> ACDVSIEGNDSMQFNTKSIVVDKTCKEFTINLKHTGKLPKAAMGHNVVVSKKSDESAVATDGMKAGLNNDYVKAGDERVIAHTSVIGGGETDSVTFDVSKLKEGEDYAFFCS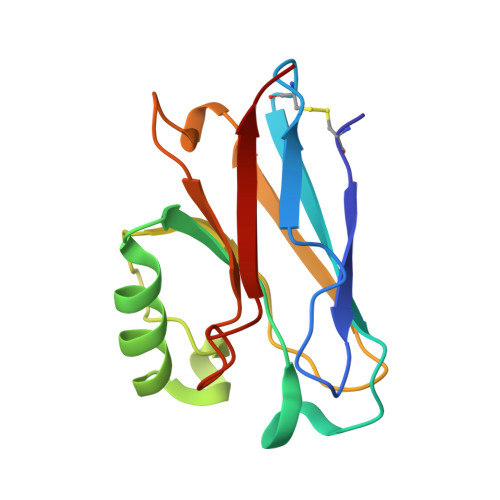FPGHWSIMKGTIELGS> GSVSMSGGFLRDDHLEFALHLHRRLAEAVPDGEVIWSPYSVACALGVLAAGARATTRTELTTLLGTDPAPLLAALDRAVTDSPDLASRTVLWVSADVPVRSSFRATMHDRPDSDVRTADFRTNPEGVRATVNADIADATRGMIRELLPQGAVTPDLRAILTNALWAKARWTTPFEAHLTRAGTFRTPRGPKRVPFMHR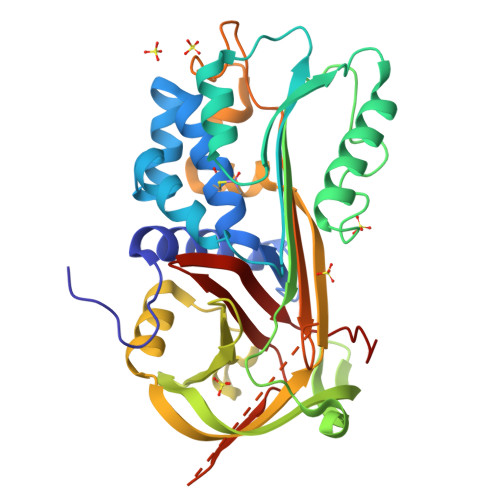TKTMPYATARGWRMVTLHAHDELAVDVLLPPGTNAAAVPTAPLLTALHRRSASTSVELALPRFELTQPHQLVEVLAEAGVRTLFTASADLSGISTVPLYVDTVIHQARLRVDERGAEGAAATAAMMLLAGAMPPRRTIRFSVDRPFHIVVRRRGAILFLGSIADPHDPGPAQ> RPPNIVLIFADDLGYGDLGCYGHPSSTTPNLDQLAAGGLRFTDFYVPVSLSTPS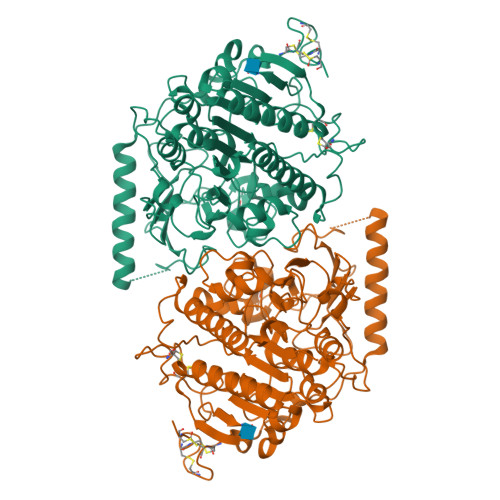RAALLTGRLPVRMGMYPGVLVPSSRGGLPLEEVTVAEVLAARGYLTGMAGKWHLGVGPEGAFLPPHQGFHRFLGIPYSHDQGPCQNLTCFPPATPCDGGCDQGLVPIPLLANLSVEAQPPWLPGLEARYMAFAHDLMADAQRQDRPFFLYYASHHTHYPQFSGQSFAERSGRGPFGDSLMELDAAVGTLMTAIGDLGLLEETLVIFTADNGPETMRMSRGGCSGLLRCGKGTTYEGGVREPALAFWPGHIAPGVTHELASSLDLLPTLAALAGAPLPNVTLDGFDLSPLLLGTGKSPRQSLFFYPSYPDEVRGVFAVRTGKYKAHFFTQGSAHSDTTADPACHASSSLTAHEPPLLYDLSKDPGENYNLLGGVAGATPEVLQALKQLQLLKAQLDAAVTFGPSQVARGEDPALQICCHPGCTPRPACCHCPDPHA>[6x]MASGGSGGVSVPALWSEVNRYGQ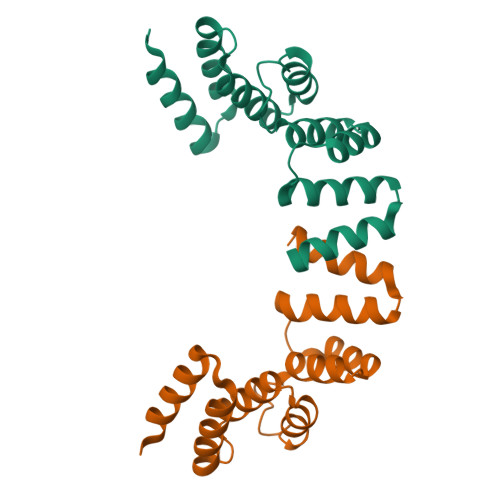NGDFTRALKTVNKILQINKDDVTALHCKVVCLIQNGSFKEALNVINTHTKVLANNSLSFEKAYCEYRLNRIENALKTIESANQQTDKLKELYGQVLYRLERYDECLAVYRDLVRNSQDDYDEERKTNLSAVVAAQSNWEK>[5x]GVYHREARSGKYKLTYAEAKAVCEFEGGHLATYKQLEAARKI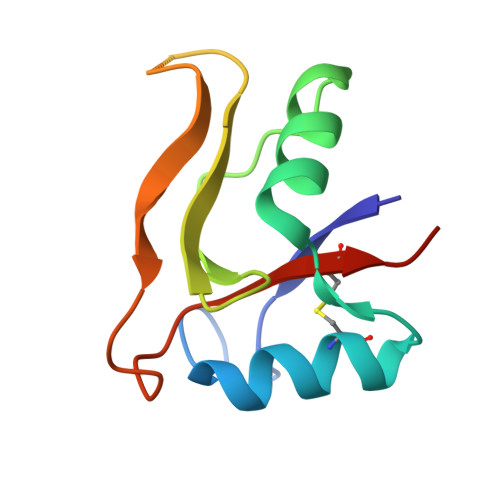GFHVCAAGWMAKGRVGYPIVKPGPNCGFGKTGIIDYGIRLNRSERWDAYCYNPHAK> MQDTDFFSWRRTMLLRFQRMETAEEVYHEIELQAQQLEYDYYSLCVRHPVPFTRPKVAFYTNYPEAWVSYYQAKNFLAIDPVLNPENFSQGHLMWNDDLFNEAQPLWE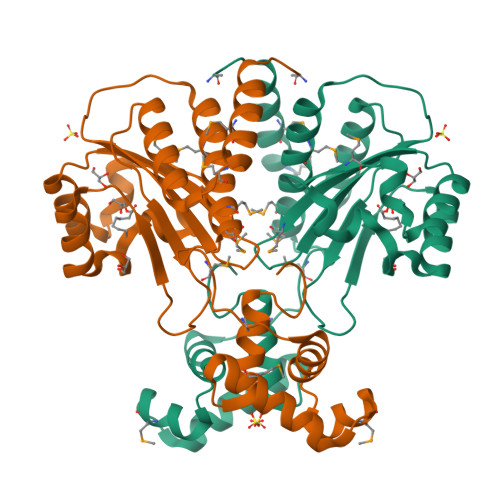AARAHGLRRGVTQYLMLPNRALGFLSFSRCSAREIPILSDELQLKMQLLVRESLMALMRLNDEIVMTPEMNFSKREKEILRWTAEGKTSAEIAMILSISENTVNFHQKNMQKKINAPNKTQVACYAAATGLIHHHHHH>SPATLPQLTPTLVSLLEVIEPEVLYAGYDSSVPDSTWRIMTTLNMLGGRQVIAAVKWAKAIPGFRNLHLDDQMTLLQYSWMFLMAFALGWRSYRQSSANLLCFAPDLIINEQRMTLP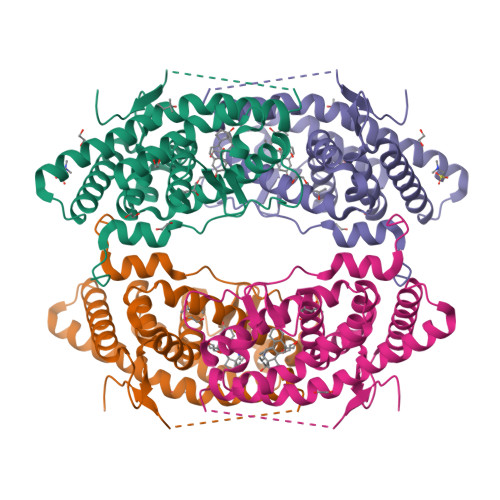CMYDQCKHMLYVSSELHRLQVSYEEYLCMKTLLLLSSVPKDGLKSQELFDEIRMTYIKELGKAIVKREGNSSQNWQRFYQLTKLLDSMHEVVENLKPYCFQTFLDKTMSIEFPEMLAEIITNQIPKYSNGNIKKLLFHQK[2x]> GPHMSRLEIYSPEGLRLDGRRWNELRRFESSINTHPHAADGSSYMEQGNNKIITLVKGPKEPRLKSQMDTSKALLNVSVNITKFSKFERSKSSHKNERRVLEIQTSLVRMFEKNVMLNIYPRTVIDIEIHVLEQDGG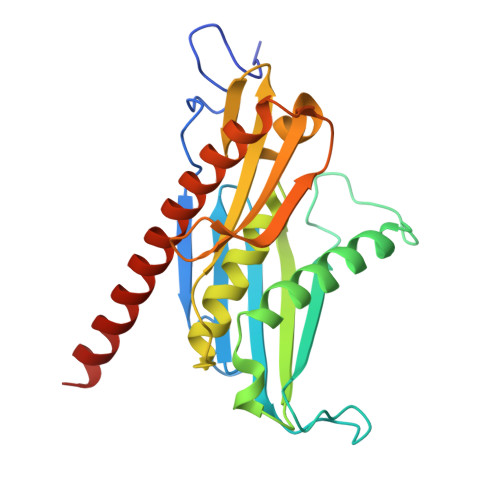IMGSLINGITLALIDAGISMFDYISGISVGLYDTTPLLDTNSLEENAMSTVTLGVVGKSEKLSLLLVEDKIPLDRLENVLAIGIAGAHRVRDLMDEELRKHAQKRVSNASAR>MRSRRVDVMDVMNRLILAMDLMNRDDALRVTGEVREYIDTVKIGYPLVLSEGMDIIAEFRKRFGCRIIADFKVADIPETNEKICRATFKAGADAIIVHGFPGADSVRACLNVAEEMGREVFLLTEMAHPGAEMFIQGAADEIARMGVDLGVKNYVGPSTRPERLSRLREI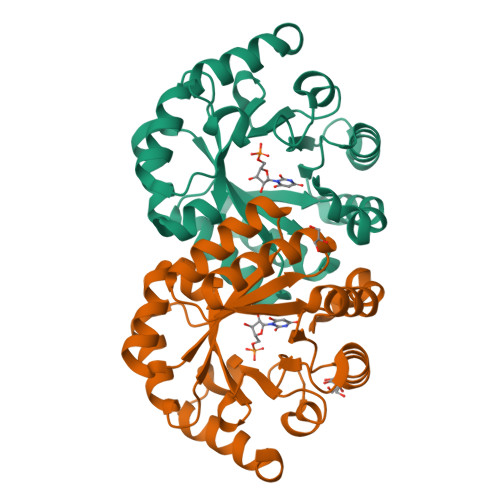IGQDSFLISPGVGAQGGDPGETLRFADAIIVGRSIYLADNPAAAAAGIIESIKDLLNP[2x]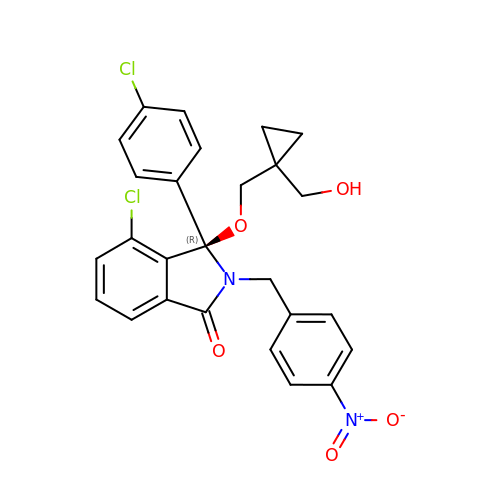(3~{R})-4-chloranyl-3-(4-chlorophenyl)-3-[[1-(hydroxymethyl)cyclopropyl]methoxy]-2-[(4-nitrophenyl)methyl]isoindol-1-one | C26 H22 Cl2 N2 O5 | DWRQUFAXBKEFJN-AREMUKBSSA-N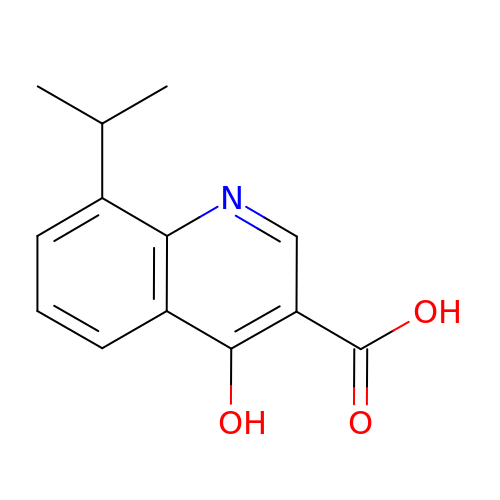4-hydroxy-8-(propan-2-yl)quinoline-3-carboxylic acid | C13 H13 N O3 | KGDOGYITTVCUJA-UHFFFAOYSA-N1-(3-{6-[(CYCLOPROPYLMETHYL)AMINO]IMIDAZO[1,2-B]PYRIDAZIN-3-YL}PHENYL)ETHANONE | C18 H18 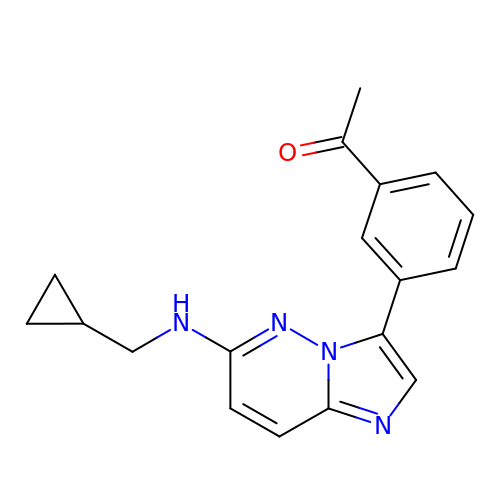N4 O | IVUBNTNWKIPCPS-UHFFFAOYSA-N> GSPGILAPLAPGSEDNFARFVCKNNGVLFENQLLQIGLKSEFRQNLGRMFIFYGNKTSTQFLNFTPTLICADDLQTNLNLQTKPVDPTVDGGAQVQQVINIECISDFTEAPVLNIQFRYGGTF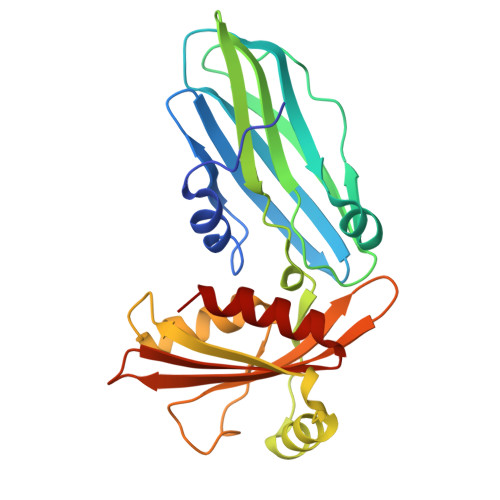QNVSVKLPITLNKFFQPTEMASQDFFQRWKQLSNPQQEVQNIFKAKHPMDTEITKAKIIGFGSALLEEVDPNPANFVGAGIIHTKTTQIGCLLRLEPNLQAQMYRLTLRTSKDTVSQRLCELLSEQF(2S)-2-[(6-azanyl-9H-purin-8-yl)sulfanyl]butanoic acid 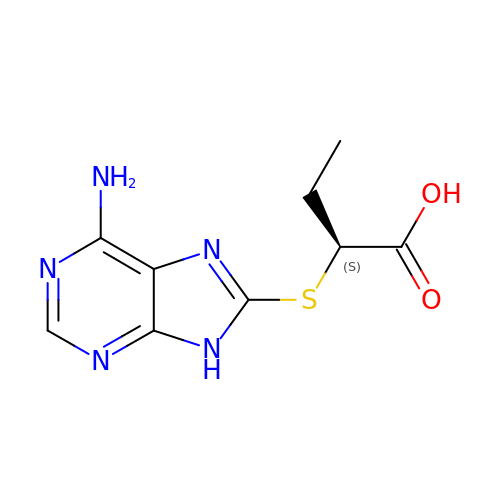| C9 H11 N5 O2 S | USXGXECUDHKQHW-BYPYZUCNSA-N>GKEELEKLAKELSKVWPELGKLVEEVIKLIEGRSKDPKAAVEGLIETMRRAADLLIEKVLELNPALKDDPARTAALVER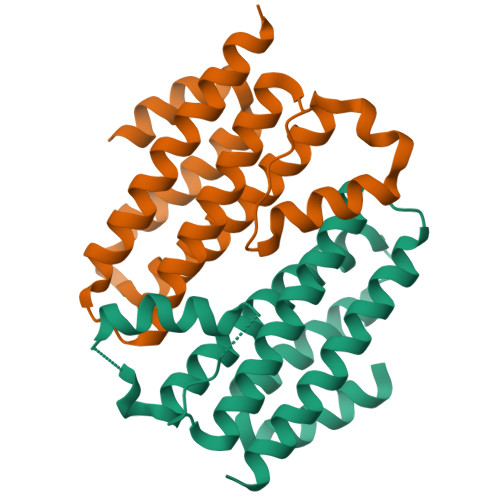LLAGTGEIPSFLSEAGRVLAEAAVAMREAADRLRAELAAGNEDLSAAADEALAVFVEAVRRVAAALLEHHHHHH[2x]Dihydroorotate dehydrogenase (DHODH) is a key enzyme in the pyrimidine biosynthesis pathway, essential for DNA and RNA syntheses in all organisms. Human DHODH (HsDHODH) belongs to class 2 DHODHs, which occur in the mitochondrial membrane and operate through a ping-pong reaction mechanism involving two distinct steps. In the first step, dihydroorotate (DHO) is oxidized to orotate (ORO) while flavin mononucleotide (FMN) is reduced. In HsDHODH, the second substrate is ubiquinone, which is reduced to ubiquinol.

The HsDHODH–lapachol complex was solved at 1.31 Å, comprising 365 residues (Thr32 to Arg396), 1 FMN molecule, 1 ORO molecule, 1 acetic acid molecule, 3 glycerol molecules, 3 sulfate ions, 1 lapachol molecule, and 245 water molecules treated as oxygens. The overall structure reveals the characteristic α-β barrel fold typical of HsDHODH structures. While this loop is often disordered in HsDHODH structures complexed with inhibitors, in the HsDHODH–lapachol complex, it is well-defined and can be reliably modeled. Lapachol binds to the N-terminal region of the enzyme, occupying the proposed ubiquinone-binding site where all currently described HsDHODH inhibitors are bound. This study discloses the first crystal structure of HsDHODH in complex with a quinone, providing strong evidence that this site is indeed the binding region for the second substrate, ubiquinone. Notably, a slight conformational change in the side chain of Arg136 observed in the crystal structure, with a root-mean-square deviation for all atoms (RMSDall) of 1.26 Å, enabled interactions with both the carbonyl group at carbon 1 and the hydroxyl group at carbon 2 of the naphthoquinone core. A minor variation in the side chain of Gln47 (RMSDall = 0.78 Å) also facilitated a hydrogen bond with the quinonoid core of lapachol in the crystal structure, a feature not predicted in the docking model. According to Baumgartner’s classification, lapachol interacts with subsites 1 (Met43, Leu46, Ala55), 2 (Arg136, Gln47), 3 (Tyr356), and 4 (Val134). Notably, the interaction with Val134 is unique to lapachol. In the crystal structure, the isoprenyl group interacts with Leu46, whereas in the predicted pose, it interacts with Leu359.

> SMATGDERFYAEHLMPTLQGLLDPESAHRLAVRFTSLGLLPRARFQDSDMLEVRVLGHKFRNPVGIAAGFDKHGEAVDGLYKMGFGFVEIGSVTPKPQEGNPRPRVFRLPEDQAVINRYGFNSHGLSVVEHRLRARQQKQAKLTEDGLPLGVNLGKNKTSVDAAEDYAEGVRVLGPLADYLVVNVSSPNTAGLRSLQGKAELRRLLTKVLQERDGLRRVHRPAVLVKIAPDLTSQDKEDIASVVKELGIDGLIVTNTTVSRPAGLQGALRSETGGLSGKPLRDLSTQTIREMYALTQGRVPIIGVGGVSSGQDALEKIRAGASLVQLYTALTFWGPPVVGKVKRELEALLKEQGFGGVTDAIGADHRR>[6x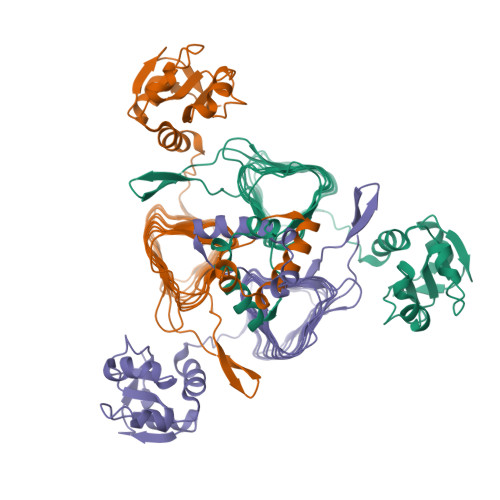]GGSKVQQYRLDELAHLVKGELIGEGSLQFSNLASLENAEVNHLTFVNGEKHLDQAKVSRAGAYIVTAALKEHLPEKDNFIIVDNPYLAFAILTHVFDKKISSTGIESTARIHPSAVISETAYIGHYVVIGENCVVGDNTVIQSHTKLDDNVEVGKDCFIDSYVTITGSSKLRDRVRIHSSTVIGGEGFGFAPYQGKWHRIAQLGSVLIGNDVRIGSNCSIDRGALDNTILEDGVIIDNLVQIAHNVHIGSNTAIAAKCGIAGSTKIGKNCILAGACGVAGHLSIADNVTLTGMSMVTKNISEAGTYSSGTGLFENNHWKKTIVRLRQLADVPLTQITKRLDHIQAQIESLESTFNLR>MSDQNNRSRNEYHSNRKNEPSYELQNAHSGLFHSSNEELTNRNQRYTNQNASMGSFTPVQSLQFPEQSQQTNMLYNGDDGNNNTINDNERDIYGGFVNHHRQRPPPATAEYNDVFNTNSQQLPSEHQYNNVPSYPLPSINVIQTTPELIHNGSQTMATPIERPFFNENDYYYNNRNSRTSPSIASSSDGYADQEARPILEQPNNNMNSGNIPQYHDQPFGYNNGYHGLQAKDYYDDPEGGYIDQRGDDYQINSYLGRNGEMVDPYDYENSLRHMTPMERREYLHDDSRPVNDGKEELDSVKSGYSHRDLGEYDKDDFSRDDEYDDLNTIDKLQFQANGVPASSSVSSIGSKESDIIVSNDNLTANRALKRSGTEIRKFKLWNGNFVFDSPISKTLLDQYATTTENANTLPNEFKFMRYQAVTCEPNQLAEKNFTVRQLKYLTPRETELMLVVTMYNEDHILLGRTLKGIMDNVKYMVKKKNSSTWGPDAWKKIVVCIISDGRSKINERSLALLSSLGCYQDGFAKDEINEKKVAMHVYEHTTMINITNISESEVSLECNQGTVPIQLLFCLKEQNQKKINSHRWAFEGFAELLRPNIVTLLDAGTMPGKDSIYQLWREFRNPNVGGACGEIRTDLGKRFVKLLNPLVASQNFEYKMSNILDKTTESNFGFITVLPGAFSAYRFEAVRGQPLQKYFYGEIMENEGFHFFSSNMYLAEDRILCFEVVTKKNCNWILKYCRSSYASTDVPERVPEFILQRRRWLNGSFFASVYSFCHFYRVWSSGHNIGRKLLLTVEFFYLFFNTLISWFSLSSFFLVFRILTVSIALAYHSAFNVLSVIFLWLYGICTLSTFILSLGNKPKSTEKFYVLTCVIFAVMMIYMIFCSIFMSVKSFQNILKNDTISFEGLITTEAFRDIVISLGSTYCLYLISSIIYLQPWHMLTSFIQYILLSPSYINVLNIYAFCNVHDLSWGTKGAMANPLGKINTTEDGTFKMEVLVSSSEIQANYDKYLKVLNDFDPKSESRPTEPSYDEKKTGYYANVRSLVIIFWVITNFIIVAVVLETGGIADYIAMKSISTDDTLETAKKAEIPLMTSKASIYFNVILWLVALSALIRFIGCSIYMIVRFFKKVTFR[2x]

Chitin is a long-chain polymer of β-(1,4)-linked N-acetylglucosamine (GlcNAc) and is synthesized by chitin synthase in the plasma membrane. In this report, we determined seven cryo-electron microscopy (cryo-EM) structures of S. cerevisiae Chs1 in the apo state and in complex with UDP-GlcNAc, UDP-GlcNAc+GlcNAc, UDP, UDP+GlcNAc, PolyB, and NikkoZ. The overall structure of Chs1 reveals a dimer architecture with a twofold symmetry and is ~100 Å tall and 110 Å wide. Each Chs1 monomer is composed of a large cytosolic soluble region and a transmembrane domain (TMD), with both the N-terminus and C-terminus in the cytosol.

Using AlphaFold2 predicted structure as initial model, we built the atomic model of Chs1 in apo state into the cryo-EM map at 2.6 Å resolution. Except for the N-terminal region and a few short loops, Chs1 is mostly ordered and well resolved. Except a short loop ranging from 245 to 271 residues, the first 374 residues of Chs1 are largely disordered and invisible in our cryo-EM maps. SDS-PAGE gel of purified Chs1-ΔSL showed the N-terminal region has been largely degradated during purification as processed by trypsin, indicating the N-terminal inhibitory region of Chs1-ΔSL is more sensitive to proteolysis. This finding is consistent with our cryo-EM map of Chs1 in apo state, which showed the segment 989-992 of swapping loop packs on segments 245-271 and 376-379 of NTR. Interestingly, we found that two phospholipid molecules fully filled this cavity and were sealed inside by EL3s. Clearly, lipids play a structural role in stabilizing the structure of the Chs1 dimer. In the apo state, the path from the active site to the chitin transmembrane channel is blocked by the VLPGA loop, in which the proline ring of P675 is stabilized by packing with the indole ring of W760. Among them, L819 of TMH1, M886 of TMH3, F911, I914, L918 of TMH4, and F1098 of TMH6 form a closed hydrophobic gate, blocking the cavity from connecting to the exoplasmic side. In the apo state of Chs1, the putative active site is open for donor binding, whereas the putative chitin transporting channel is sealed by a switch loop in cytosolic side and TMH4 in exoplasmic side.> GIGTGFPFDPHYVEVLGERMHYVDVGPRDGTPVLFLHGNPTSSYVWRNIIPHVAPTHRCIAPDLIGMGKSDKPDLGYFFDDHVRFMDAFIEALGLEEVVLVIHAWGSALGFHWAKRNPERVKGIAF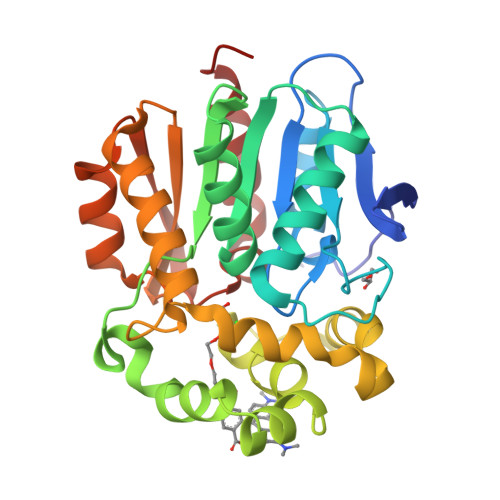MEFIRPIPTWDEWPEFARETFQAFRTTDVGRKLIIDQNVFIEGTLPMGVVRPLTEVEMDHYREPFLNPVDREPLWRFPNELPIAGEPANIVALVEEYMDWLHQSPVPKLLFWGTPGVLIPPAEAARLAKSLPNCKAVDIGPGLNLLQEDNPDLIGSEIARWLSTLEI> GSMLDFSKDFLFGVATASYQVEGAYNEDGRTMSIWDTFSRQDGKVYKSHNGDVACDHYHLYKDDVKMMKDLGIEAYRFSIAWPRIFPAKGQYNPKGMDFYKRLTDELLKNDIKPFATIYHWDLPQWADDLGGWLNREIVEWYGEYAEKLFSELGGYIKNWITLNEPWCSSFLSYFIGEHAPGHKDLGEALLVSHNLLLSHGKAVEIFRGLNLDDSKIGITLNLNEVFPASDSDDDKVAAQIADGFQNRWFLDPLFKGKYPQDMVEYFGKYAKVDFINDEDLKLISQKLDFLGVNYYTRAVVQKGNDGLLDAVQIDPGNERTEMGWEIYPESLYNILMRLKREYTYDMPLYITENGAAFNDVVEDDGRVHDEKRVEFLKQHFKEAKRFLNDGGNLKGYFVWSLMDNFEWAHGYSKRFGIVYVDYETEKRILKDSALWYKDLISTRTI

β-Glucosidases (Bgls) convert cellobiose and other soluble cello-oligomers into glucose and play important roles in fundamental biological processes, providing energy sources in living organisms. Bgls are essential terminal enzymes of cellulose degradation systems and attractive targets for lignocellulose-based biotechnological applications. In this study, we report the biochemical and structural analysis of a Bgl from the hemicellulose-degrading thermophilic anaerobe Thermoanaerobacterium saccharolyticum (TsaBgl). Bgl cleaves β-1,4-glycosidic linkages in disaccharides and glucose-substituted polysaccharides and is involved in the utilization of polysaccharides as an energy source in cells.

To better elucidate the molecular function of TsaBgl, we determined the crystal structure of TsaBgl at 1.70 Å resolution. Crystals of TsaBgl belonged to the orthorhombic space group P212121 with one molecule per asymmetric unit. TsaBgl contained 16 α-helices and 13 β-strands, forming a single (β/α)8 TIM-barrel fold with dimensions of 55 × 55 × 50 Å. The conserved active site containing the crucial residues Glu163 (proton donor) and Glu351 (nucleophile), which are involved in the acid-base mechanism, is located in the center of the TIM-barrel. Temperature factor analysis showed that the core of the TIM-barrel of TsaBgl was highly rigid, whereas the loop between the β8-strand and α14-helix (named the β8-α14 loop) showed structural flexibility and was ~20 Å away from the substrate-binding entrance. During the structure refinement, strong Fo-Fc electron density was observed in the active site pocket corresponding to the Tris molecule of the buffer solution, which was characterized as an inhibitor in our biochemical study. Analysis of the crystal structure of TsaBgl showed that one Tris molecule is bound to the glycone site and interacted with Glu163 and Glu351, which are involved in the hydrolytic activity of TsaBgl. The binding configuration of the Tris molecule in the active site of TsaBgl was similar to those in the structures TreBgl, ManBgl, and HthBgl, whereas the structures OsaBgl, SfrBgl, and ubBgl showed distinct binding configurations of Tris. The enzyme activity of TsaBgl was significantly inhibited by the Tris molecule. To better understand glucose recognition of TsaBgl, we performed a soaking experiment to bind glucose to TsaBgl; however, in all crystal structures, Tris, not glucose, was bound to the active site, indicating that glucose had lower binding affinity than Tris.> MVFGTLYTFPGDQCRTIAIKAVAKANGLDLDIRETPRTPDHLSISKLGKVPAFQGADSFKLFECMAIALYITSQNEQTTLLGKDKKEYAEIIKWMSFFNTEIVILMTQQLLPQLGVIPYDRDQVEFFANMTQRSVDVVEEYLQDRTFLVGDQLSLADLFCAGNISLGFQFFYGKAWRQQNPNVSRWYEMVCHQPIYAAVTDKFQLLDEPKLTNNPPE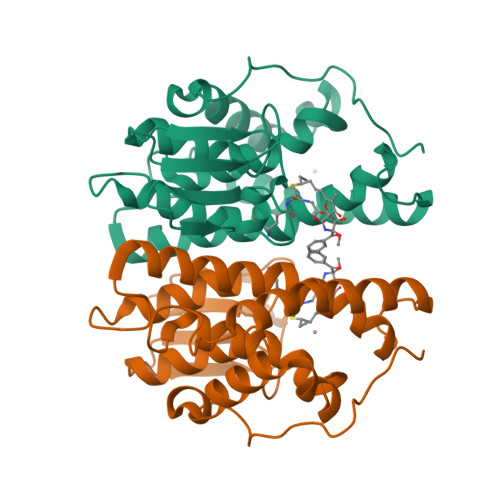KKPETVPKNGAAVAIEATQAGHHHHHH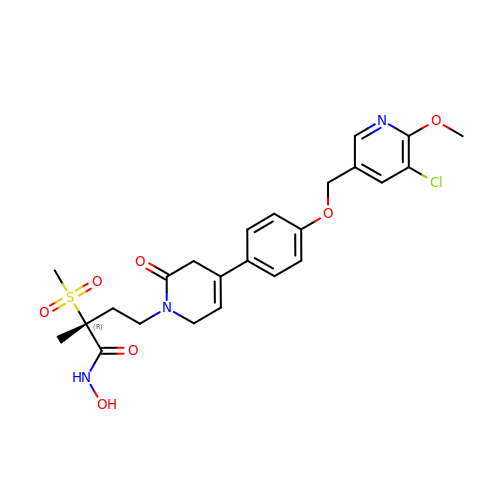(2R)-4-[4-{4-[(5-chloro-6-methoxypyridin-3-yl)methoxy]phenyl}-2-oxo-3,6-dihydropyridin-1(2H)-yl]-N-hydroxy-2-methyl-2-(methylsulfonyl)butanamide | C24 H28 Cl N3 O7 S | CDFIGPHKVBKXMP-XMMPIXPASA-N>HGYIKEPVSRAYMGALEKQTMGWTAAAQKYGSVIDNPQSVEGPKGFPAAGPPDGRIASANGGSGQIDFGLD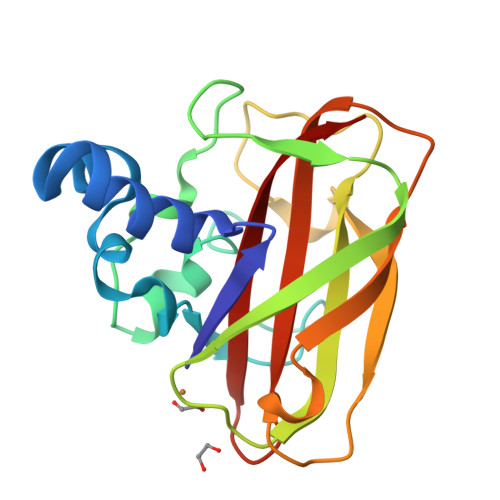KQTADHWVKQNIRGGFNTFTWHYTAPHATSKWHYYITKKNWNPNKPLSRDEFELIGTVNHDGSKADTNLTHKIFVPTDRSGYHIILGVWDVADTSNAFYNVIDVNLT[2x]> MSDDLVKILVLGPSKSGKSTVTNFLAGTRDTPTKEYHETNPLRVLEVEIALDDTRRSGRQAAGLKKAVVQLWDVGGSSKHQAGWPAIASNADGIIYVFNPEVKGSEKELLLWYKNFALNQDELDDDNNFKMRVTDGHSLIFSHHSSLPEFAVGDNAIPPMPPKQLQGIRALET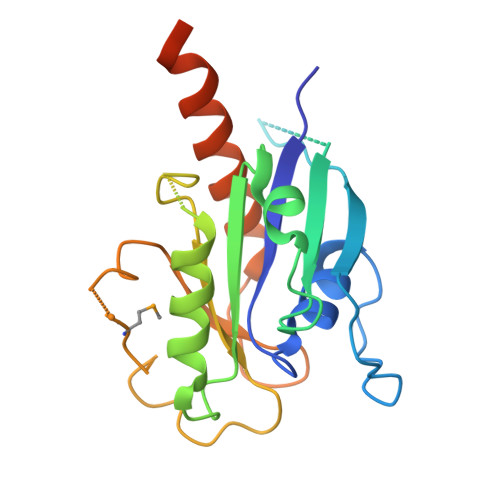SLDYQSDNFKEAFDALVEQIIASRLAAEENDLLQKEREAKDYPRLKR(4~{S})-5-[4-[[4-(2-ethyl-2-oxidanyl-butoxy)-3-methyl-phenyl]-dipropyl-silyl]-2-methyl-phenoxy]-4-oxidanyl-pentanoic 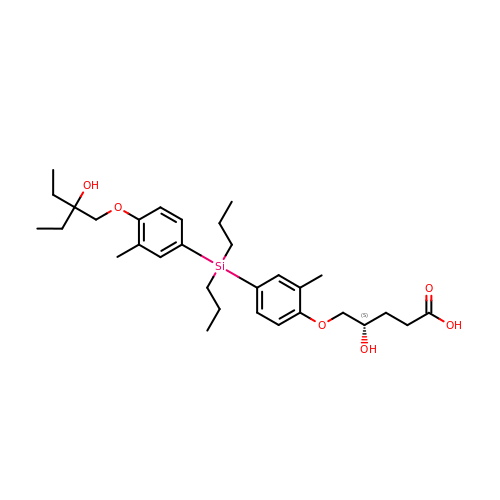acid | C31 H48 O6 Si | WEFOCDOWLUCQPS-VWLOTQADSA-N> KK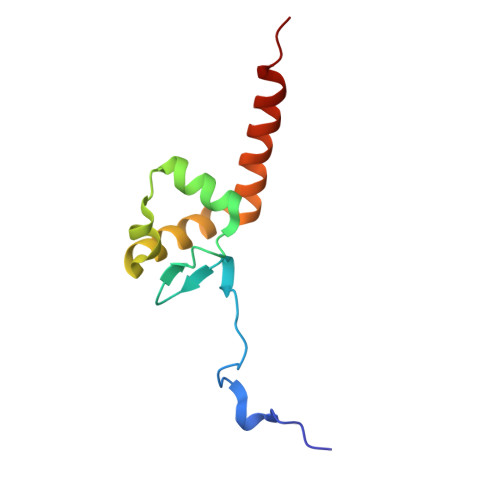KRLTKADIGTPSNFQHIGHVGWDPNTGFDLNNLDPELKNLFDMCGISEAQLKDRETSKVIYDFIEKTGGVEAVKNELRRQAENLYFQGLEH>[4x]MAIELLYDADADLSLIQGRKVAIVGYGSQGHAHSQNLRDSGVEVVIGLREGSKSAEKAKEAGFEVKTTAEAAAWADVIMLLAPDTSQAEIFTNDIEPNLNAGDALLFGHGLNIHFDLIKPADDIIVGMVAPKGPGHLVRRQFVDGKGVPCLIAVDQ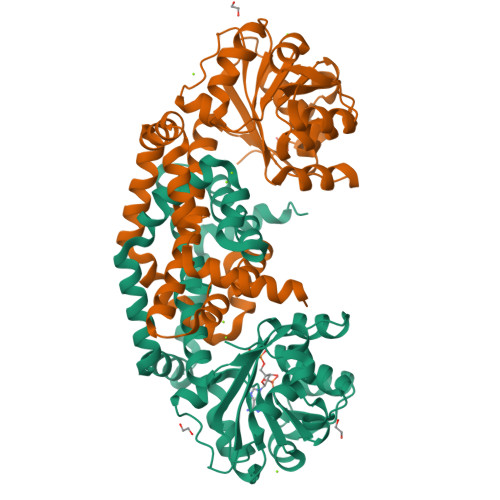DPTGTAQALTLSYAAAIGGARAGVIPTTFEAETVTDLFGEQAVLCGGTEELVKVGFEVLTEAGYEPEMAYFEVLHELKLIVDLMFEGGISNMNYSVSDTAEFGGYLSGPRVIDADTKSRMKDILTDIQDGTFTKRLIANVENGNTELEGLRASYNNHPIEETGAKLRDLMSWVKVDARAETAHHHHHH N-methyl-1-[(4-methylbenzyl)sulfonyl]methanamine | C10 H15 N O2 S | 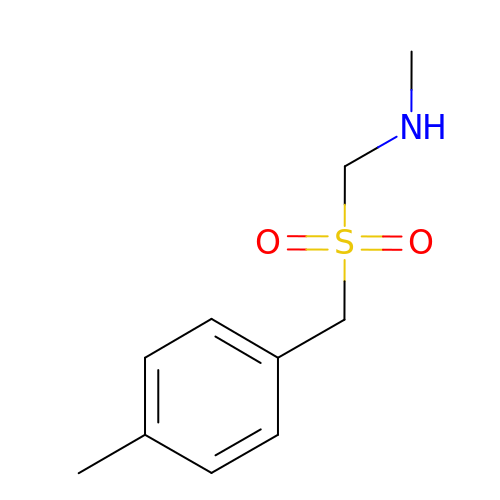XASGHCUSPMUTIK-UHFFFAOYSA-N>MKDIAIRGYCDRPSVATGETIRFYVSANETRGTFDAELVRLIHGDSNPAGPGYKEEAIKSDLEGQYPARFQRTQFGSYVEVADPDAGLQPDGAFSVHLFLWSTTPSRGRQGIASRWNDERQSGWNLAIEDGRVVFTIGDGSGATSSVVSDRPLFQQIWYSITGVYDPEKKQLRLYQKSVVNRTNSRFGLVVPLDSDCAVSADATVKAADSETSLLIAGLGEAAAQDGRTWCIAHYNGKVDAPKIYGCALGQDDAEKLSRGEIVRPISRLAHWDFSAGIGLNGIPTDHVVDASGYGHHGRCMNQPSRGSTGWNWDGHEENFIHCPEQYGALWFHEDCLDDCRWEKDFEFTVPEGLKSDFYAVKIRYEDTEDYIPFFVLPPRGTATAPILVIASTLSYLAYANEQIMHKADIGQAVAGHTPVLNENDVELHKNLSYYGLSTYDGHIDGRGVQYTSWRRPIMNLRPKHRQGFGSIWELPADLHLIDWLNHNGFEYDVATEHDLNDQGAELLRRYKVVLTGSHPEYQTWANADAWEDYLADGGRGMYLAANGMYWIVEVHPEKPWVMEVRKELGVTAWEAPPGEYHYSTNGRRGGRFRGRARATQKIWGTGMSSFGFDHSGYFVQMPDSQDERVAWIMEGIDPEERIGDGGLVGGGAGGYELDRYDLALGTPPNTLLLASSVEHSVVYTVIPDDKAFPHPGMNGGEHPFVRADITYFSTANGGGMFATSSISWLGSLSWNDYDNNVSKMTKNVLNQFIKDEPAPRVKLAAALEHHHHHH[8x];>MTEASESCVRDPSNYRDRSADWYAFYDERRRKEIIDIIDEHPEIVEEHAANPFGYRKHPSPYLQRVHNYFRMQPTFGRYYIYSEREWDAYRIATIREFGELPELGDERFKTEEEAMHAVFLRRIEDVRAELA[8x]

Certain bacterial species from genera such as Paracoccus, Pseudomonas, and Alcaligenes have evolved to use DMF as a sole carbon and nitrogen source for growth via degradation by a dimethylformamidase (DMFase). We show that DMFase from Paracoccus sp. strain DMF is a halophilic and thermostable enzyme comprising a multimeric complex of the α2β2 or (α2β2)2 type. The active site consists of a mononuclear iron coordinated by two Tyr side‐chain phenolates and one carboxylate from Glu. The Fe3+ ion in the active site catalyzes the hydrolytic cleavage of the amide bond in DMF.

The overall structure from both these techniques is similar. The exact nature of the metal ion as Fe was confirmed by X‐ray fluorescence spectroscopy at the synchrotron. The mononuclear Fe atom is tetra‐coordinated with the protein. It is coordinated to two phenolates of tyrosine residues (Y399 and Y440 serve as monodentate ligands), and a glutamic acid carboxylate side chain (E521 serves as a bidentate ligand).>[4x]GHMHPLLRRLDLNLLLV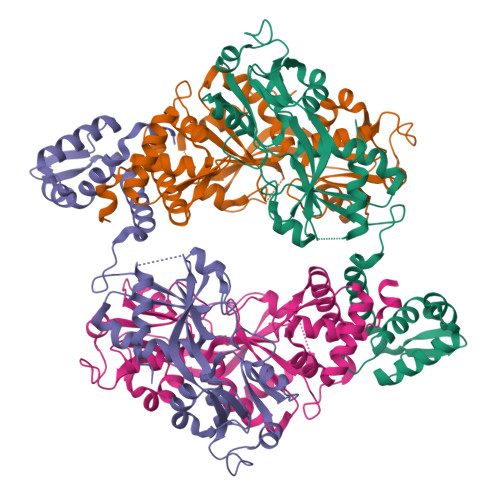FDALYRHRNVGTAASELAISASAFSHALGRLRQGLDDELFLRQGNRMQPTQRAEHLAAAVAAALRALGEGLEEWRPFVPGQSQRTFVFAATDYTAFALLPPLMNRLQHSAPGVRLRLVNAERKLSVEALASGRIDFALGYDEEHERLPEGIQAHDWFADRYVVVARRDHPRLAGAPTLEGYLAERHAVVTPWNEDSGVIDRLLARSGLRREVAVQLPTVLAALFLAGSTDFLLTAPRHAARALAEAAGLALYPAPFDIPPYVLRLYSHVQHVGRDAHAWMIGQLKGLDISRTG> VSFPASVQLHTAVEMHHWCIPFSVDGQPAPSLRWLFNGSV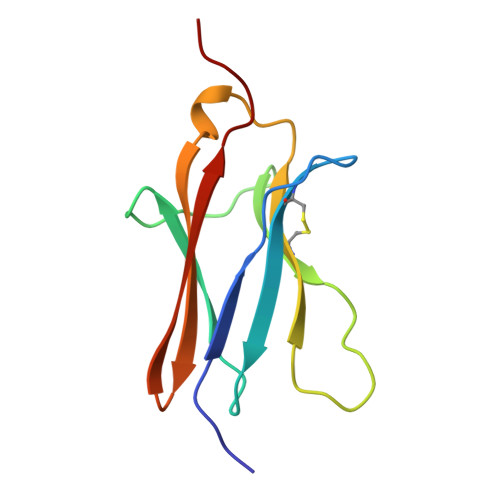LNETSFIFTEFLEPAANETVRHGCLRLNQPTHVNNGNYTLLAANPFGQASASIMAAFMDNP4-{3-[4-(1,1,1,3,3,3-hexafluoro-2-hydroxypropan-2-yl)benzyl]-2,2-dioxido-2,1,3-benzothiadiazol-1(3H)-yl}-N-[(2R)-4-hydroxybutan-2-yl]-N-methylbutanamide 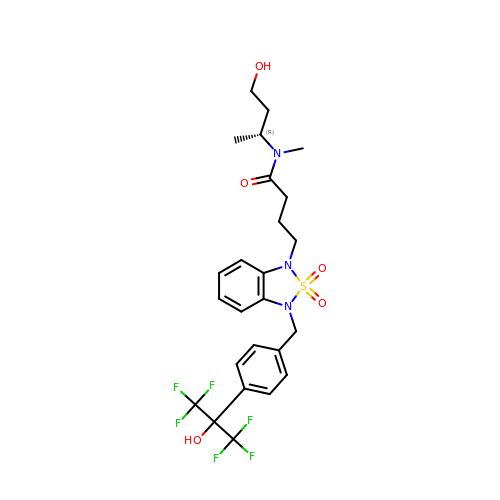| C25 H29 F6 N3 O5 S | SULHDXFOLGGHOR-QGZVFWFLSA-N> MSTAVQFRGGTTAQHATFTGAAREITVDTDKNTVVVHDGATAGGFPLARHDLVKTAFIKADKSAVAFTRTGNATASIKAGTIVEVNGKLVQFTADTAITMPALTAGTDYAIYVCDDGTVRADSNFSAPTGYTSTTA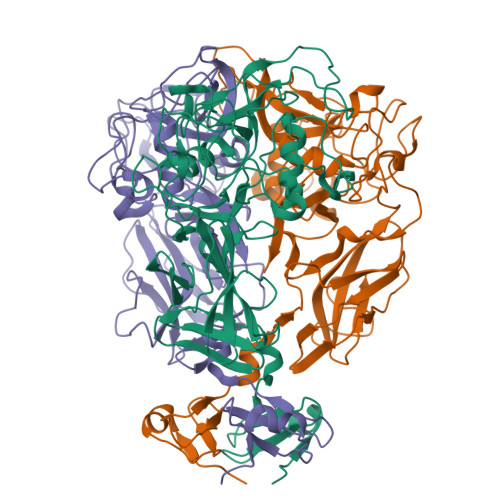RKVGGFHYAPGSNAAAQAGGNTTAQINEYSLWDIKFRPAALDPRGMTLVAGAFWADIYLLGVNHLTDGTSKYNVTIADGSASPKKSTKFGGDGSAAYSDGAWYNFAEVMTHHGKRLPNYNEFQALAFGTTEATSSGGTDVPTTGVNGTGATSAWNIFTSKWGVVQASGCLWTWGNEFGGVNGASEYTANTGGRGSVYAQPAAALFGGSWFYTSYSGSRAAYWNAGPSNSSANIGARGVCDHLILE> SRRNLGAGHWKSPKGKVDPRAGWQNGKQTGSGCGPNECKGLPNRHLIRPPYMIQNGAGPTLADSTADTDLVQSGGYVQYDTHNLYGAMMSSHSHNAMRARRPDDRALVITRSTFAGSGKDVSHWLGDNVSGWLWYQLSISQILQFASLYQIPVVGPDVCGFGGNVTETLCARWATLGSFYTFFRNHAEIYANPQEFYRWPTVAQAARNGISIRYQLLDYIYTAIYKQNQTGTPALNPLFFNYPNDPNTYPIDLQFFYGDGILVSPVTEENSTSVT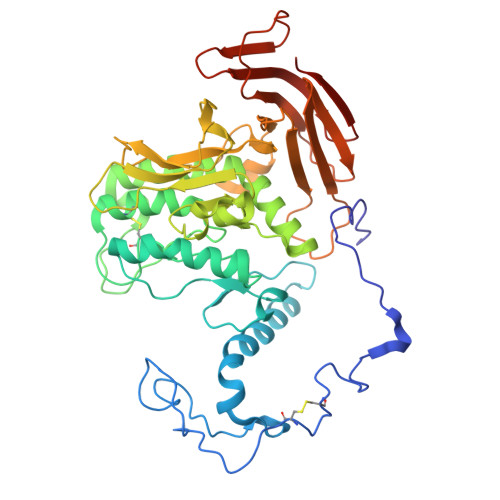FYLPDDIFYEWGTGKPVRGQGEYVSLDNIDYTDITIHYKGGIVYPQRIESANTTTALRQKGFNIVVAPGLDGRAEGSLYLDDGVSVVQDTVSEIDFVYENGKLTMTGSFEYEAGVGIETITVLGVESKPEGDEDVEYDAENKKLVKHVDVPLTGENEITILAVDHHHHHH>[2x]MGSYDSSSSSSNDSSARNEEDESCMFALKLLGGFAVPFTIKAVIELGVMDQLLTAERAMSAEELVAAAVAAQLPRPEVACTMVDRLLRFLASHSVVRCTTEVVVGTDDATTTTCCRRSYAASPVCKWFARNGVEDSVLPLGMMILNKTFLDSWQNITDAVLEGAAPFEKTYGMPMFEYLSTNGPLNTVFHEAMANHSMIITKKLLKFFRGFEGLD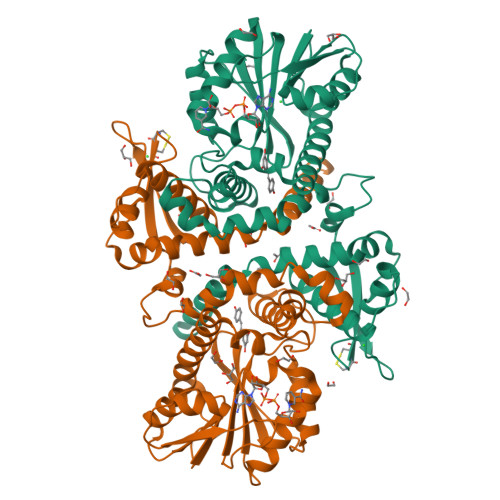VLVDVGGGNGTTLQMIRGQYKNMRGINYDLPHVIAQAAPVEGVEHVGGSMFDNIPRGNAVLLKWILHDWDDKACIKILKNCYTALHVRGKVIVLEYVVPDEPEPTLAAQGAFELDLTMLVTFGSGKERTQREFSELAMEAGFSREFKATYIFANVWALEFTK4-(2,4-DICHLOROPHENOXY)-2'-METHYLBIPHENYL-3-OL 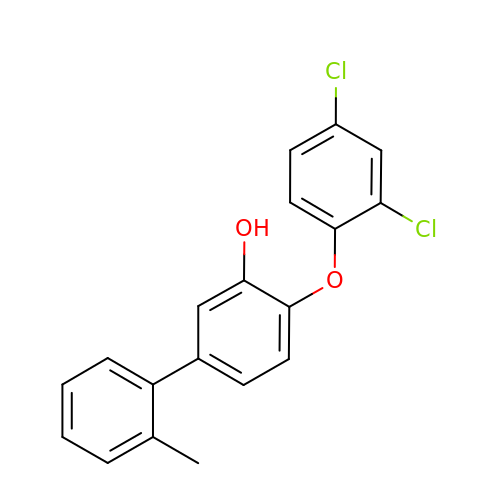| C19 H14 Cl2 O2 | VDWAWADVXJMBAA-UHFFFAOYSA-N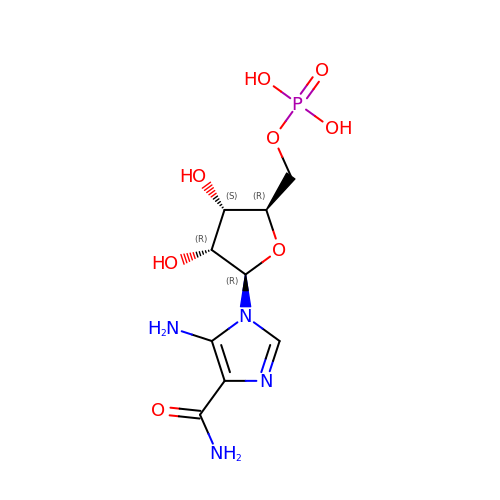AMINOIMIDAZOLE 4-CARBOXAMIDE RIBONUCLEOTIDE | C9 H15 N4 O8 P | NOTGFIUVDGNKRI-UUOKFMHZSA-N> GAGEARLEEAVNRWVLKFYFHEALRAFRGSRYGDFRQIRDIMQALLVRPLGKEHTVSRLLRVMQCLSRIEEGENLDCSFDMEAELTPLESAINVLEMIKTEFTLTEAVVESSRKLVKEAAVIICIKNKEFEKASKILKKHMSKDPTTQKLRNDLLNIIREKNLAHPVIQNFSYETFQQKMLRFLESHLDDAE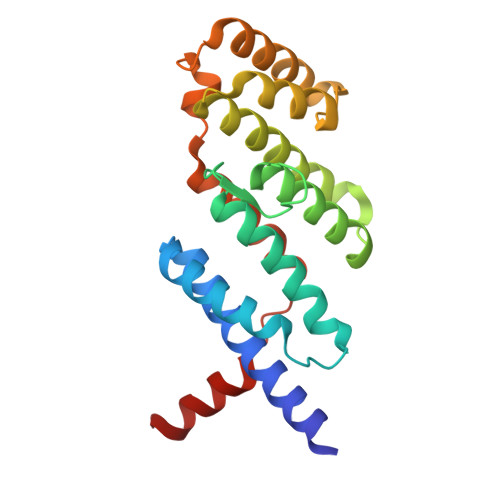PYLLTMAKKALK>MSGETTRLTEPQLRELAARGAAELDGATATDMLRWTDETFGDIGGAGGGVSGHRGWTTCNYVVASNMADAVLVDLAAKVRPGVPVIFLDTGYHFVETIGTRDAIESVYDVRVLNVTPEHTVAEQDELLGKDLFARNPHECCRLRKVVPLGKTLRGYSAWVTGLRRVDAPTRANAPLVSFDETFKLVKVNPLAAWTDQDVQEYIADNDVLVNPLVREGYPSIGCAPCTAKPAEGADPRSGR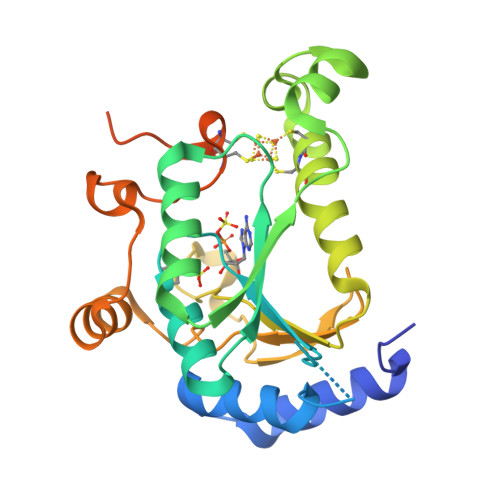WQGLAKTECGLHASLEHHHHHH[2x]> GPLGSEAHLYMQVQIVAEDQFCGHQGNDMYDEEKVKYTVFKVLKNSSLAEFVQSLSQTMGFPQDQIRLWPMQARSNGTKRPAMLDNEADGNKTMIELSDNENPWTIFLETVDPELAASGATLPKFD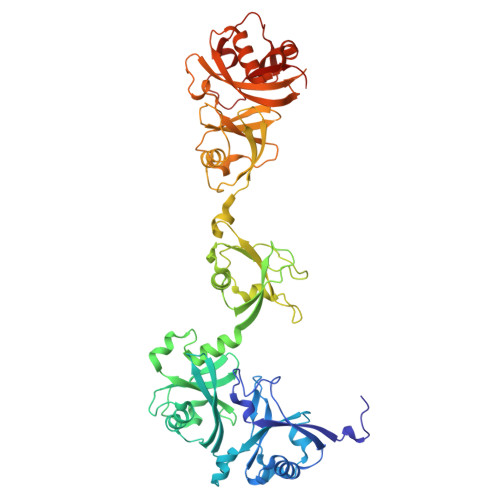KDHDVMLFLKMYDPKTRSLNYCGHIYTPISCKIRDLLPVMCDRAGFIQDTSLILYEEVKPNLTERIQDYDVSLDKALDELMDGDIIVFQKDDPENDNSELPTAKEYFRDLYHRVDVIFCDKTIPNDPGFVVTLSNRMNYFQVAKTVAQRLNTDPMLLQFFKSQGYRDGPGNPLRHNYEGTLRDLLQFFKPRQPKKLYYQQLKMKITDFENRRSFKCIWLNSQFREEEITLYPDKHGCVRDLLEECKKAVELGEKASGKLRLLEIVSYKIIGVHQEDELLECLSPATSRTFRIEEIPLDQVDIDKENEMLVTVAHFHKEVFGTFGIPFLLRIHQGEHFREVMKRIQSLLDIQEKEFEKFKFAIVMMGRHQYINEDEYEVNLKDFEPQPGNMSHPRPWLGLDHFN> A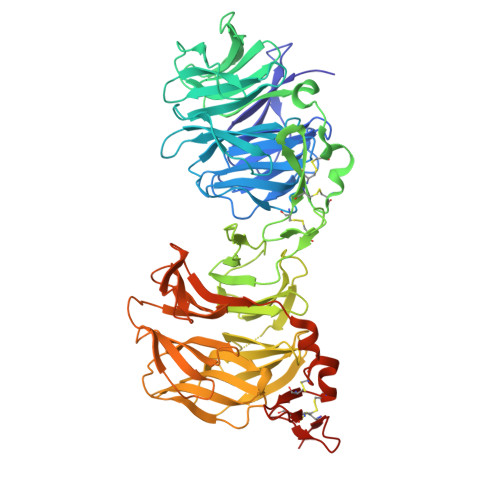DPEAFLLFSRRADIRRISLETNNNNVAIPLTGVKEASALDFDVTDNRIYWTDISLKTISRAFMNGSALEHVVEFGLDYPEGMAVDWLGKNLYWADTGTNRIEVSKLDGQHRQVLVWKDLDSPRALALDPAEGFMYWTEWGGKPKIDRAAMDGSERTTLVPNVGRANGLTIDYAKRRLYWTDLDTNLIESSNMLGLNREVIADDLPHPFGLTQYQDYIYWTDWSRRSIERANKTSGQNRTIIQGHLDYVMDILVFHSSRQSGWNECASSNGHCSHLCLAVPVGGFVCGCPAHYSLNADNRTCSAPTTFLLFSQKSAINRMVIDEQQSPDIILPIHSLRNVRAIDYDPLDKQLYWIDSRQNMIRKAQEDGSQGFTVVVSSVPSQNLEIQPYDLSIDIYSRYIYWTCEATNVINVTRLDGRSVGVVLKGEQDRPRAIVVNPEKGYMYFTNLQERSPKIERAALDGTEREVLFFSGLSKPIALALDSRLGKLFWADSDLRRIESSDLSGANRIVLEDSNILQPVGLTVFENWLYWIDKQQQMIEKIDMTGREGRTKVQARIAQLSDIHAVKELNLQEYRQHPCAQDNGGCSHICLVKGDGTTRCSCPMHLVLLQDELSCGEPHHHHHHHHHH(2S,3S)-3-FORMYL-2-({[(4-NITROPHENYL)SULFONYL]AMINO}METHYL)PENTANOIC ACID | C13 H16 N2 O7 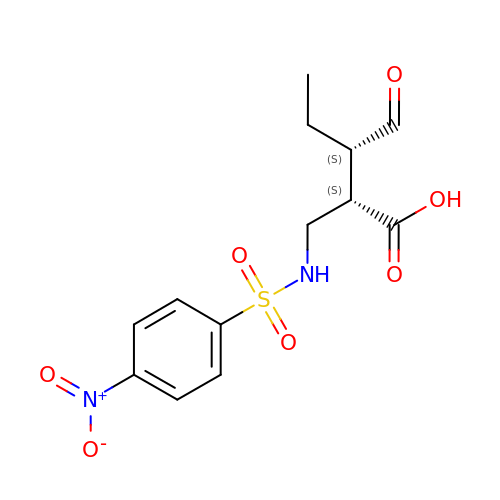S | JPQYVEFTAZEPOD-BXKDBHETSA-N> SALFEPYTLKDVTLRNRIAIPPMCQYMAEDGMINDWHHVHLAGLARGGAGLLVVEATAVAPEGRITPGCAGIWSDAHAQAFVPVVQAIKAAGSVPGIQIAHAGRKASANRPWEGDDHIAADDTRGWETIAPSAIAFGAHLPKVPREMT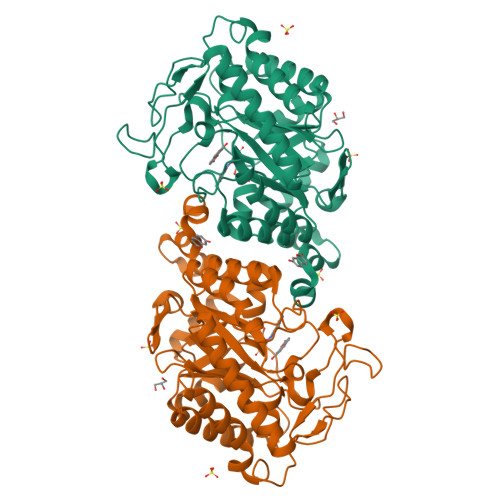LDDIARVKQDFVDAARRARDAGFEWIELHFAHGFLGQSFFSEHSNKRTDAYGGSFDNRSRFLLETLAAVREVWPENLPLTARFGVLEYDGRDEQTLEESIELARRFKAGGLDLLSVSVGFTIPDTNIPWGPAFMGPIAERVRREAKLPVTSAWGFGTPQLAEAALQANQLDLVSVGRAHLADPHWAYFAAKELGVEKASWTLPAPYAHWLE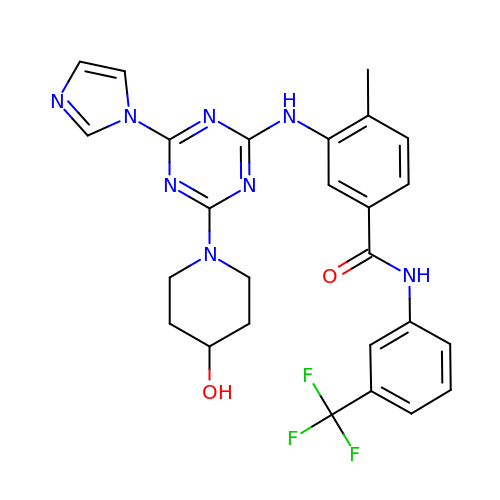3-[[4-imidazol-1-yl-6-(4-oxidanylpiperidin-1-yl)-1,3,5-triazin-2-yl]amino]-4-methyl-~{N}-[3-(trifluoromethyl)phenyl]benzamide | C26 H25 F3 N8 O2 | ZHVJHWWEVILTJQ-UHFFFAOYSA-N>[5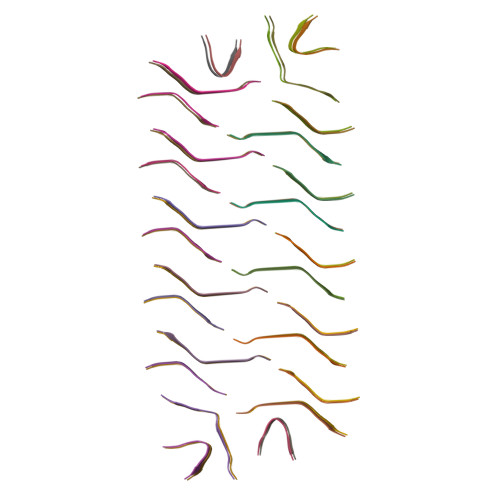2x]GPLGMLGGVVIA5-(6-D-RIBITYLAMINO-2,4-DIHYDROXYPYRIMIDIN-5-YL)-1-PENTYL-PHOSPHONIC ACID | C14 H26 N3 O9 P | 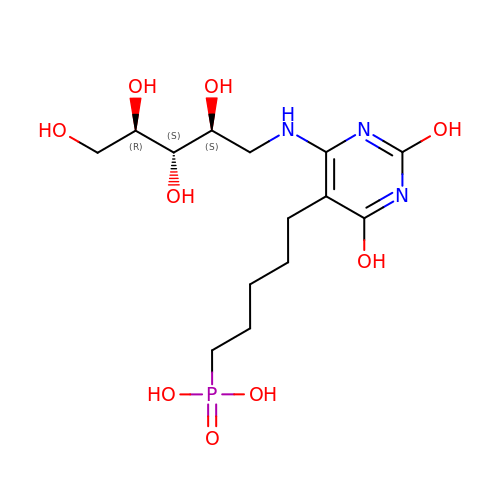BMATWAHJJFXMFA-AXFHLTTASA-N>[2x]MQLFHKAINRRGTHSIKWDTYKNEELIHAWIADMDFEVPKPIQTALKQRIKHPIFGYTLPPENIGDIICNWTKQQYDWDIQKEWIVFSAGIVPALSTSIQAFTKENESVLVQPPIYPPFFEMVTTNNRQLCVSPLQKQNDTYVIDFKHLEKQFQQGIKLMLLCSPHNPIGRVWTKEELIKLGSLCTKYNVIVVADEIHSDIIYADHTHTPFASLSEELAERTITCMA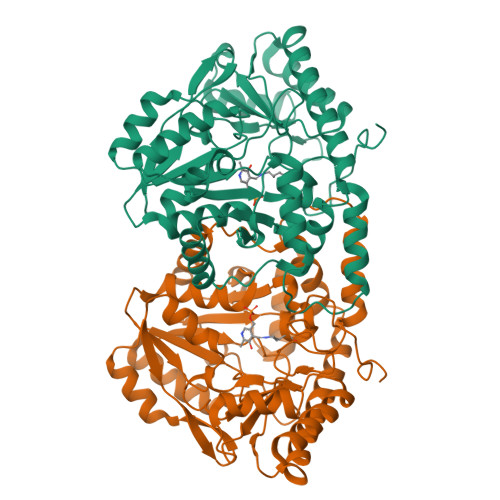PSKTFNIAGLQASIIIIPNEKLRHAFTAIQYRQGFHGLNIFAYTAMQSAYTECNDWLNKIRLYIEDNAKFACEYMKDHIPTLSVTKPEGSFLLWIDCSALNLSQDERTKLLEEKGKIIVEPGEKYGLGGEEHIRINIGCPRSVLEEILNRLRHTFS>MAASGEPQRQWQEEVAAVVVVGSCMTDLVSLTSRLPKTGETIHGHKFFIGFGGKGANQCVQAARLGAMTSMVCKVGKDSFGNDYIENLKQNDISTEFTYQTKDAATGTASIIVNNEGQNIIVIVAGANLLLNTEDLRAAANVISRAKVMVCQLEITPATSLEALTMARRSGVKTLFNPAPAIADLDPQFYTLSDVFCCNESEAEILTGLTVGSAADAGEAALVLLKRGCQVVIIT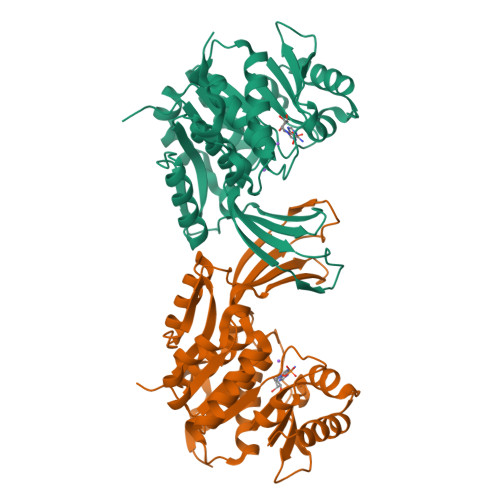LGAEGCVVLSQTEPEPKHIPTEKVKAVDTTGAGDSFVGALAFYLAYYPNLSLEDMLNRSNFIAAVSVQAAGTQSSYPYKKDLPLTLFLEHHHHHH[2x]>[3x]GCSSGVRCWATRQAMLGQVHEVPEGWLIFVAEQEELYVRVQNGFRKVQLEARTPLPR

We describe the development of a biologic that takes advantage of the proximity of the N-terminus of bound ACE2 to the three-fold symmetry axis of the spike protein to create an ultrapotent, trivalent ACE2 entry antagonist. Therefore, we sought trimeric scaffolds to fuse three ACE2 moieties and leverage the inherent symmetry of the spike trimer to maximize avidity. Thus, we determined a trimeric antagonist fused to the N-terminus of ACE2 would require a short peptide linker and would be less likely to form inter-spike interactions. The collagen VIII trimerization domain is significantly larger than the collagen XVIII domain (44.7 kDa and 19.3 kDa, respectively), but more importantly, previous studies reported that collagen VIII melts at ~45 °C66, whereas the collagen XVIII domain melts at ~85 °C (vide infra). Given these observations, the smaller, more thermally stable collagen XVIII trimerization domain was advanced to develop the trimeric antagonist.

We then sought to prevent the dissociation of the collagen XVIII trimer via the introduction of intermolecular disulfide bonds, despite the high reported trimerization constant (where 50% of the trimer is monomeric) of 56 pM49. Cysteine mutations capable of creating inter-chain disulfide associations (i.e., C®-C® distances less than 6 Å and absence of obvious steric clashes) were identified: G22–F'26, E31–V'37, and G(-1)–L’5. The parental construct yielded ~1.7 mg·L−1 purified protein (n = 1); the disulfide mutants, E31C–V'37C and G(-1)C–L’5C constructs, yielded each ~1 mg·L−1 protein each (n = 1); whereas the G22C–F'26C mutant only yielded ~0.05–0.2 mg·L−1 protein (n = 2). The formation of inter-chain disulfide bonds was confirmed by X-ray diffraction studies. High-resolution crystal structures of the E31C–V'37C and G(-1)C–L’5C mutants afforded clear electron density for the disulfide bonds in both mutants (respectively). Furthermore, the thermal stability of each collagen disulfide mutant was assessed by DSF. The ‘wildtype’ collagen XVIII trimerization domain produced a calculated melting temperature of 84.9 ± 0.2 °C. However, two of the disulfide mutants (G(-1)C–L’5C and E31C–V'37C) either produced very low or no fluorescent intensity up to 100 °C. Considering the high melting temperature of the “parental” collagen XVIII, we posit that the melting temperatures of the disulfide mutants exceed 100 °C. Given the poor expression of the G22C–F'26C mutant with our trimeric ACE2 constructs, we proceeded with E31C–V'37C.> QNKELCDVTSSTGLLDSIKVMASHVKEQLKDKGTSEVAQPIVSPDPTDCADILLNGYRSSGGYRIWPKSWMTVGTLNVYCDMETDGGGWTVIQRRGNYGNPSDYFYKPWKNYKLGFGNIEKDFWLGNDRIFALTNQRNYMIRFDLKDKENDTRYAIYQDFWIENEDYLYCLHIGNYSGDAGN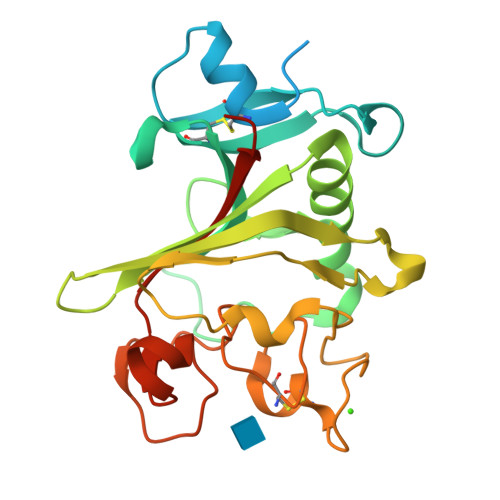SFGRHNGHNFSTIDKDHDTHETHCAQTYKGGWWYDRCHESNLNGLYLNGEHNSYADGIEWRAWKGYHYSLPQVEMKIRPVEFNIIGN> GNEPSDLLEAEQIEKLAKHLPPRTIGYPWNLAFSTSKHGMS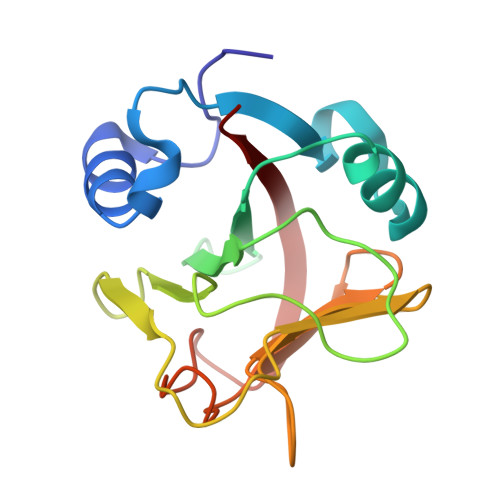IKTLYRAMQDQDSPMLLVIKDSDGQIFGALASEPFKVSEGFYGTGETFLFTFYPEFEAYKWTGDNLFFIKGDMDSLAFGGGSGEFGLWLDGDLYHGRNHSCKTFGNPMLSMKEDFFVQDIEIWSFE> GPLGSAKATVEQLMFEEKNKAQRLQTELDVSEQVQ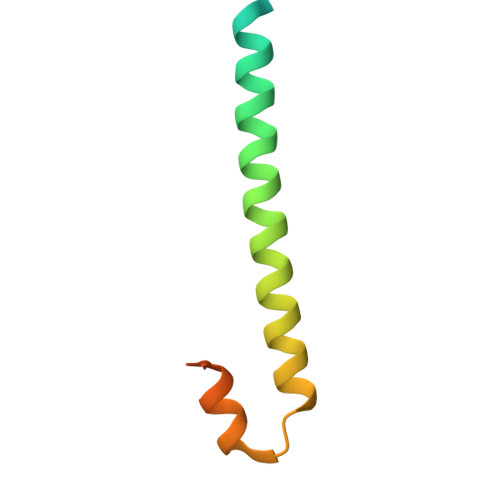RDFVKLSQTLQVQLERIRQADSLERIRAILNDTKLTDINQLPET>[8x]MDKIYIHDMEFYGYHGVFPEENKLG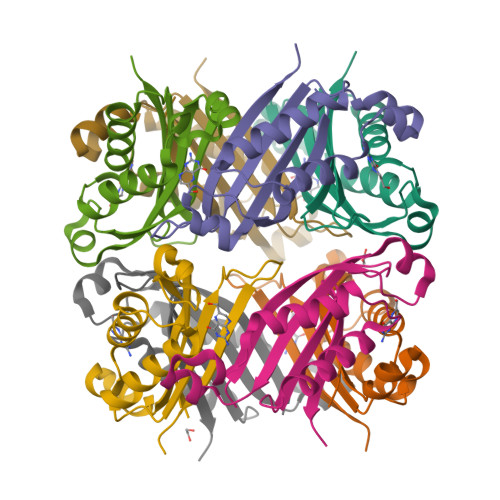QRFKVDLTVELDLKRAGESDDLEHSVNYGELFELCRKVVEDRTYKLVESIAENIATDILKQYESISRCTIKVIKPDPPIPGHYRAVAVEITRERP>[4x]GDITHMASMTGGQQMGRDPMRICSFNVRSFGESKQEDKNAMDVIVKVIKRCDIILVMEIKDSNNRICPILMEKLNRNSRRGITYNYVISSRLGRNTYKEQYAFLYKEKLVSVKRSYHYHDYQDGDADVFSREPFVVWFQSPHTAVKDFVIIPLHTTPETSVKEIDELVEVYTDVKHRWKAENFIFMGDFNAGCSYVPKKAWKNIRLRTDPRFVWLIGDQEDTTVKKSTNCAYDRIVLRGQEIVSSVVPKSNSVFDFQKAYKLTEEEALDVSDHFPVEFKLQ

The enzymes responsible for clearing antigenic DNA from serum have been identified as Dnase1 and Dnase1L3 (deoxyribonuclease 1 like 3 or Dnaseγ); yet, the activities assigned to these two enzymes are not synonymous. Dnase1L3 uniquely degrades antigenic forms of cell-free DNA, including DNA complexed with lipids and proteins. Dnase1 and Dnase1L3 are both Ca2+/Mg2+-dependent endonucleases with a high degree of identity in the active site; however, the catalytic mechanism of the Dnase1-family remains contested.

Full-length Dnase1L3 was refractory to crystallization, likely because of the flexible C-terminus; therefore, we expressed and purified a form of Dnase1L3 missing the last 23 residues (ΔCTD) for the structural analysis of the core domain. Dnase1L3 ΔCTD was crystallized at pH 8.5 in 250 mM MgCl2 in the P1 triclinic space group with four Dnase1L3 ΔCTD molecules in the asymmetric unit. The core Dnase1L3 enzyme was refined to a final resolution of 2.2 Å with an R-free of 23%. The crystal structure of Dnase1L3 exhibits the classic 4-layer α-β sandwich architecture similar to other members of the exo/endo phosphatase (EEP) family of enzymes. The Dnase1L3 core enzyme structure superimposes with human Dnase110 with an RMSD of 1.8 Å across all C-α atoms. In Dnase1L3, we observed three divalent cations, with two Mg2+ present within the catalytic site. Our high-resolution crystal structure of Dnase1L3 provides the first experimental support for the two-cation catalytic mechanism, wherein His-155 and His-274 act as the catalytic acid and base residues, respectively. Using the nomenclature from Guéroult, the ’II’ and ’III’ structural cations are absent in Dnase1L3. In the Dnase1L3 crystal structure, which lacks DNA, Arg-132 interacts with His-155 to decrease the pKa of His-155 favoring the deprotonated form. In addition to the previously predicted Glu-170 to Arg-206 salt bridge, our structural analysis shows that Arg-206 forms an extensive salt-bridged network with Asp-166 and Glu-167.Diltiazem | C22 H26 N2 O4 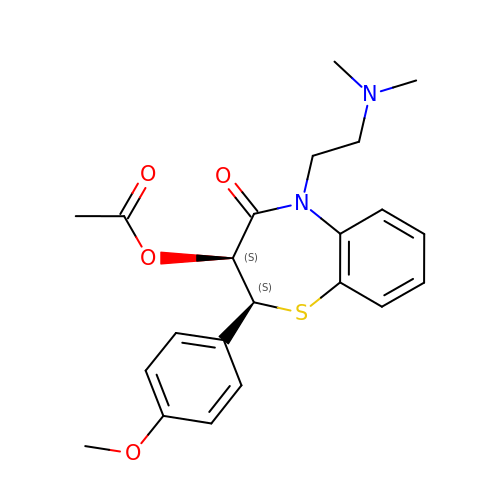S | HSUGRBWQSSZJOP-RTWAWAEBSA-N>GSELAHFQSEIEENYEAVGNVVVDLMGGCEPTLRVGRVQLGNDIFTLREEIRATELKRVLYVGTTEGDEFPVVVYAWTNGNSYESAKAFVASQGLNVPCRIVGYRSYDKMSGYTAIIFPQGHVYSLRTFLQRSVPTRATETALYYVAETLRSLCTRRIIHCALTP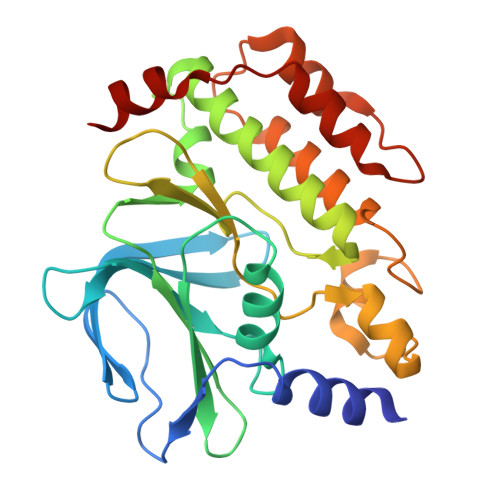DNVFMYMDSTGASLKTFPVCWDDCVDAAMFSERGLKFVPSLPVLMRHAVKEIDGSYIDFVSFCRMFRQIENNCSAMCQKVAKMKAPPVVRMTDYTNIQTELTWDMDAVMNHFC[2x]> SDRLIQITRGDSTITSQDTANAVVAYGVWPSYLTPDDATAIDKPTQPDTSSNRFYTLDSRSWTSASSGWWWKLPDALKNMGIFGENMFYHFLGRSGYTIHVQCNSSKFHQGLLIVAAIPEHQLASATSGNVSV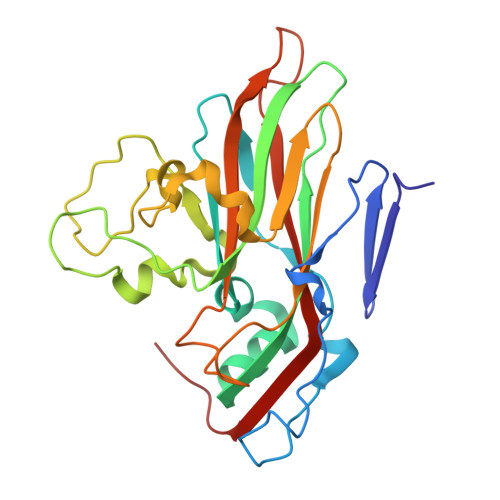GYNHTHPGEQGREVVPSRTSSDNKRPSDDSWLNFDGTLLGNLPIYPHQYINLRTNNSATLILPYVNAVPMDSMLRHNNWSLVIIPICPLQVQPGGTQSIPITVSISPMFSEFSGPRSKVVF> SMRRIVVTGMGMINSLGLNKEDSFLAIAKGECGIKHIESFDASAFPVRIAGEITDFDPTEVMNPKDVKKAGRFIQLALKATREAMKDSGILDAHNRCPEELANRMGVSSGSGIGGLGNIEANSIFCFEKGPRKVNPFFITSALVNMIG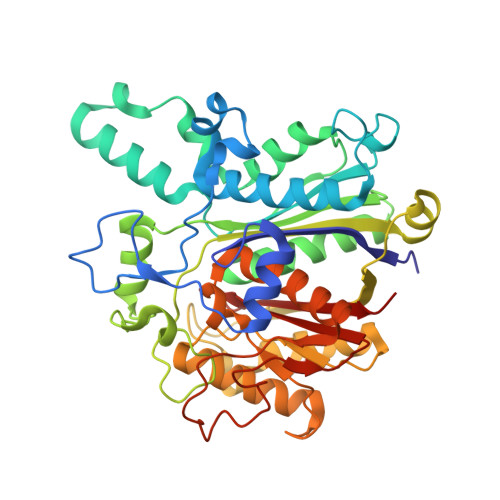GFTSIEFGIKGPNLSSVTACAAGTHAIIEAVKTILLNGADRMLVVGAESTICPVGIGGFASIKALSTRNDEPKKASRPFDKDRNGFVMGEGAGALVLEEYESAKKRGAKIYAEFAGYGESGDANHITAPAPEGEGAFRAMKMALEMAKVEVGYVNAHGTSTHYNDLYESIALKNVFGSKEKVPPVSSTAGQIGHCLGAAGALEAVISIMAMNQGILPPTINQETPDPECDLDYIPNAAREKQVDAVMSNSFGFGGTNGVVIFKKA>TQKPHLGNAGDSVTLNDVANVMYYGEAQIGDNKQKFAFIFDTGSANLWVPSAQCNTIGCKTKNLYDSNKSKTYEKDGTKVEMNYVSGTV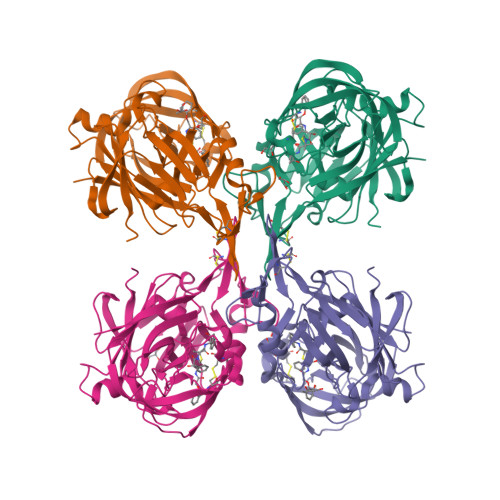SGFFSKDIVTIANLSFPYKFIEVTDTNGFEPAYTLGQFDGIVGLGWKDLSIGSVDPVVVELKNQNKIEQAVFTFYLPFDDKHKGYLTIGGIEDRFYEGQLTYEKLNHDLYWQVDLDLHFGNLTVEKATAIVDSGTSSITAPTEFLNKFFEGLDVVKIPFLPLYITTCNNPKLPTLEFRSATNVYTLEPEYYLQQIFDFGISLCMVSIIPVDLNKNTFILGDPFMRKYFTVFDYDNHTVGFALAKKKL[4x]> MSMLGERRRGLTDPEMAAVILKALPEAPLDGNNKMGYFVTPRWKRLTEYEALTVYAQPNADWIAGGLDWGDWTQKFHGGRPSWGNETTELRTVDWFKHRDPLRRWHAPYVKDKAEEWRYTDRFLQGYSADGQIRAMNPTWRDEFINRYWGAFLFNEYGLFNAHSQGAREALSDVTRVSLAFWGFDKIDIAQMIQLERGFLAKIVPGFDESTAVPKAEWTNGEVYKSARLAVEGLWQEVFDWNESAFSVHAVYDALFGQFVRREFFQRLAPRFGDNLTPFFINQAQTYFQIAKQGVQDLYYNCLGDDPEFSDYNRTVMRNWTGKWLEPTIAALRDFMGLFAKLPAGTTDK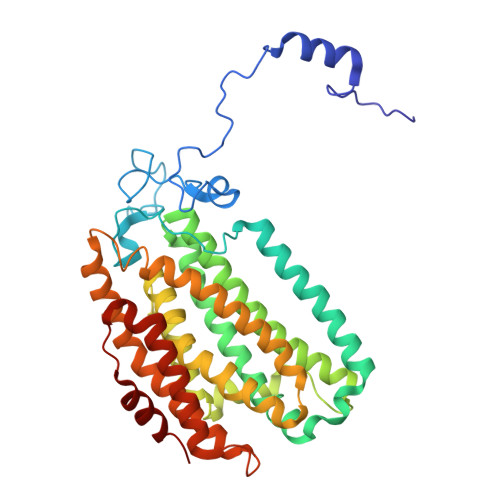EEITASLYRVVDDWIEDYASRIDFKADRDQIVKAVLAGLK> VVGGLVALRGAHPYIAALYWGHSFCAGSLIAPCWVLTAAHCLQDRPAPEDLTVVLGQERRNHSCEPCQTLAVRSYRLHEAFSPVSYQHDLALLRLQEDADGSCALLSPYVQPVCLPSGAARPSETTLCQVAGWGHQFEGAEEYASFLQEAQVPFLSLERCSAPDVHGSSILPGMLCAGFLEGGTDACQGDSGGPLVCEDQAAERRLTLQG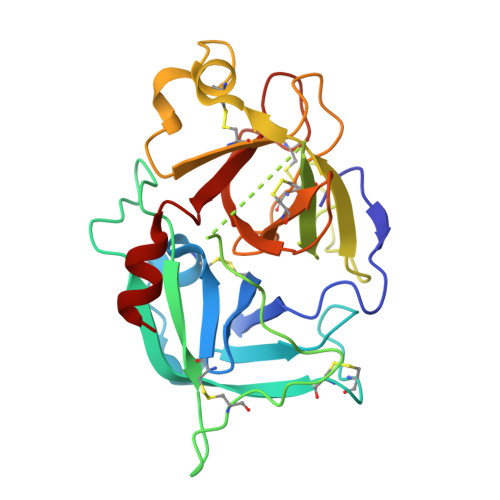IISWGSGCGDRNKPGVYTDVAYYLAWIREHT>MLGAIAYTGNKQSLLPELKSHFPKYNRFVDLFCGGLSVSLNVNGPVLANDIQEPIIEMYKRLINVSWDDVLKVIKQYKLSKTSKEEFLKLREDYNKTRDPLLLYVLHFHGFSNMIRINDKGNFTTPFGKRTINKNSEKRFNHFKQNCDKIIFSSLHFKDVKILDGDFVYVDPPYLITVADYNKFWSEDEEKDLLNLLDSLNDRGIKFGLSNVLEHHGKENTLLK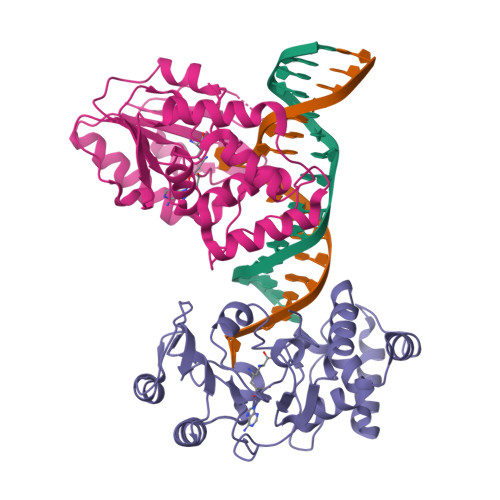EWSKKYNVKHLNKKYVFNIYHSKEKNGTDEVYIFN[4x]>MAGFWVGTAPLVAAGRRGRWPPQQLMLSAALRTLKHVLYYSRQCLMVSRNLGSVGYDPNEKTFDKILVANRGEIACRVIRTCKKMGIKTVAIHSDVDASSVHVKMADEAVCVGPAPTSKSYLNMDAIMEAIKKTRAQAVHPGYGFLSENKEFARCLAAEDVVFIGPDTHAIQAMGDKIESKLLAKKAEVNTIPGFDGVVKDAEEAVRIAREIGYPVMIKASAGGGGKGMRIAWDDEETRDGFRLSSQEAASSFGDDRLLIEKFIDNPRHIEIQVLGDKHGNALWLNERECSIQRRNQKVVEEAPSIFLDAETRRAMGEQAVALARAVKYSSAGTVEFLVDSKKNFYFLEMNTRLQVEHPVTECITGLDLVQEMIRVAKGYPLRHKQADIRINGWAVECRVYAEDPYKSFGLPSIGRLSQYQEPLHLPGVRVDSGIQPGSDISIYYDPMISKLITYGSDRTEALKRMADALDNYVIRGVTHNIALLREVIINSRFVKGDISTKFLSDVYPDGFKGHMLTKSEKNQLLAIASSLFVAFQLRAQHFQENSRMPVIKPDIANWELSVKLHDKVHTVVASNNGSVFSVEVDGSKLNVTSTWNLASPLLSVSVDGTQRTVQCLSREAGGNMSIQFLGTVYKVNILTRLAAELNKFMLEKVTEDTSSVLRSPMPGVVVAVSVKPGDAVAEGQEICVIEAMKMQNSMTAGKTGTVKSVHCQAGDTVGEGDLLVELE[6x];>[6x]MAAALRVAAVGARLSVLASGLRAAVRSLCSQATSVNERIENKRRTALLGGGQRRIDAQHKRGKLTARERISLLLDPGSFVESDMFVEHRCADFGMAADKNKFPGDSVVTGRGRINGRLVYVFSQDFTVFGGSLSGAHAQKICKIMDQAITVGAPVIGLNDSGGARIQEGVESLAGYADIFLRNVTASGVIPQISLIMGPCAGGAVYSPALTDFTFMVKDTSYLFITGPDVVKSVTNEDVTQEELGGAKTHTTMSGVAHRAFENDVDALCNLRDFFNYLPLSSQDPAPVRECHDPSDRLVPELDTIVPLESTKAYNMVDIIHSVVDEREFFEIMPNYAKNIIVGFARMNGRTVGIVGNQPKVASGCLDINSSVKGARFVRFCDAFNIPLITFVDVPGFLPGTAQEYGGI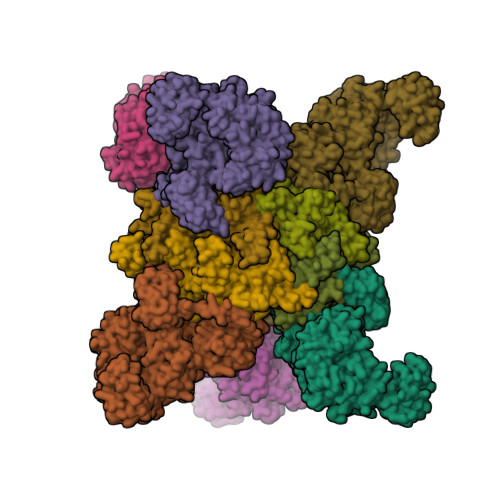IRHGAKLLYAFAEATVPKVTVITRKAYGGAYDVMSSKHLCGDTNYAWPTAEIAVMGAKGAVEIIFKGHENVEAAQAEYIEKFANPFPAAVRGFVDDIIQPSSTRARICCDLDVLASKKVQRPWRKHANIPL>TADTDRAYLEINLNNLEHNVNTLQKAMSPKCELMAVVKAEAYGHGMYEVTTYLEQIGVSSFAVATIDEGIRLRKYGISSEILILGYTSPSRAKELCKYELTQTLIDYRYSLLLNKQGYDIKAHIKIDTGMHRLGFSTEDKDKILAAFSLKHIKVAGIFTHLCAADSLEENDVAFTNKQIGSFYKVLDWLKSSGLNIPKVHIQSSYGLLNYPEL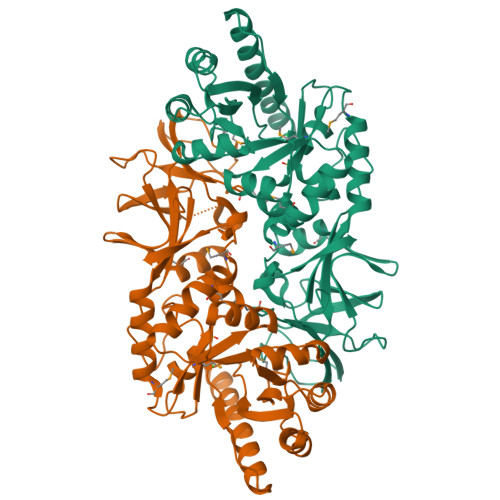ECDYIRVGVALYGVLSSTNDKTKLELDLRPVLSLKAKVVLIRKIKQGESVGYSRAFTATRDSLIAILPIGYADGFPRNLSCGNSYVLIGGRQAPIVGKICMDQLAVDVTDIPNVKTGSIATLIGKDGKEEITAPMVAESAESITNELLSRMGHRLNIIRRA[4x]>MKIAVMTDSTSYLSQDLIDKYNIQIAPLSVTFDDGKNFTESNEIAIEEFYNKMASSQTIPTTSQPAIGEWITKYEMLRDQGYTDIIVICLSSGISGSYQSSYQAGEMVEGVNVHAFDSKLAAMIEGCYVLRAIEMVEEGYEPQQIIDDLTNMREHTGLYLIVDDLKNLQKSGRITGAQAWVGTLLKMKPVLKFEDGKIIPEEKVRTKKRAIQTLEKKVLDIVKDFEEVTLFVINGDHFEDGQALYKKLQDDCPSAYQVAYSEFGPVVAAHLGSGGLGLGYVGRKIRLT[2x]

Staphylococcus aureus FakB1 is a prototypical bacterial FA transfer protein that binds palmitate within a narrow, buried tunnel. Here, we use a combination of X-ray crystallography, NMR spectroscopy, MD simulations, site-directed mutagenesis, and functional biochemical assays to characterize the membrane-bound conformation of FakB. This study focuses on FakB1, an FA transfer protein from S. aureus that binds palmitic acid (16:0) before presenting it to FakA for phosphorylation and exchange with the membrane. The bacterial class of FA transfer proteins is called FakB, and the bound acyl chains are completely enclosed within the protein interior. The open conformation arises from a conformational change in the dynamic region that rotates helix α8 outward to uncover the FA-binding tunnel and reorganizes the adjacent α8-β9 loop into a new amphipathic helix.

We identified two alanine residues (121 and 158) in the tunnel and mutated them to bulkier residues to partially occlude the FA-binding pocket and push the FA out of its pocket to destabilize the fully closed FakB1 conformation. We also determined the 2.33 Å crystal structure of FakB1(A158L), which was structurally identical to FakB1(A121I). The open FakB1(A158L) molA structure superimposes on the FakB1(A121I) molA structure with an RMSD of 0.265 Å. A similar process occurs in FakB1(A158L). First, compared with the wild-type protein, the thermal stabilities of FakB1(A121I) and FakB1(A158L) were reduced by 6 °C and 4 °C, respectively, showing that the mutations indeed prevent FakB1 from adopting its most stable conformation. When expressed in Escherichia coli, the total amount of FA incorporated by the FakB1 mutant proteins was the same as the wild-type protein, but FakB1 only supported the incorporation of palmitic acid (16:0), whereas both mutant proteins were less specific and also incorporated oleate (18:1) and linoleate (18:2). The FakB1(A121I) and FakB1(A158L) crystal structures capture the open conformation that is generated by the introduction of bulkier side chains into the FA-binding pocket and stabilized by the crystal packing architecture that creates a surrogate hydrophobic environment that favors the formation of helix α8′.>[2x]SNQAKADAVKEAFQHAWNGYMKYAFPHDELTPVSNGHADSRNGWGASAVDALSTAVIMGKADVVNAILEHVADIDFSKTSDTVSLFETTIRYLAGMLSGY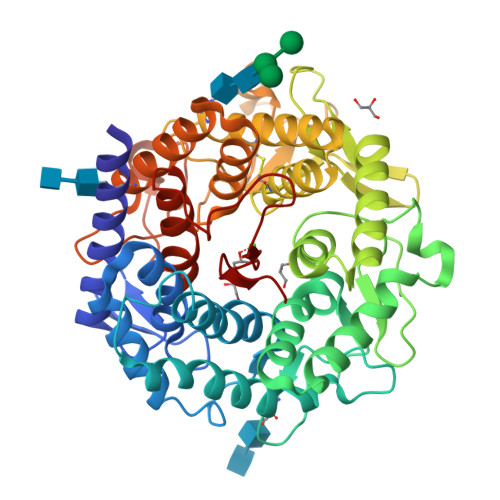DLLQGPAKNLVDNQDLIDGLLDQSRNLADVLKFAFDTPSGVPYNNINITSHGNDGATTNGLAVTGTLVLEWTRLSDLTGDEEYAKLSQKAESYLLKPQPSSSEPFPGLVGSSININDGQFADSRVSWNGGDDSFYEYLIKMYVYDPKRFETYKDRWVLAAESTIKHLKSHPKSRPDLTFLSSYSNRNYDLSSQHLTCFDGGSFLLGGTVLDRQDFIDFGLELVDGCEATYNSTLTKIGPDSWGWDPKKVPSDQKEFYEKAGFYISSGSYVLRPEVIESFYYAHRVTGKEIYRDWVWNAFVAINSTCRTDSGFAAVSDVNKANGGSKYDNQESFLFAEVMKYSYLAHSEDAAWQVQKGGKNTFVYNTEAHPISVAR> PPE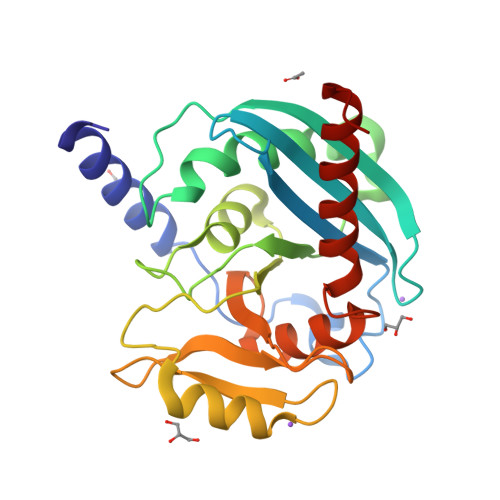ETLSLWKREQARLKAHVVDRDTEAWQRDPAFSGLQRVGGVDVSFVAGDSVRACASLVVLSFPELEVVYEESRMVSLTAPYVSGFLAFREVPFLLELVQQLREKEPGLMPQVLLVDGNGVLHHRGFGVASHLGVLTDLPCVGVAKKLLQVDGLANNALHKEKIRLLQTRGDSFPLLGDSGTVLGMALRSHDRSTRPLYISVGHRMSLEAAVRLTSACSRFRIPEPVRQADICSREHIRKSLGLP>[2x]GAMDPEFALQELRAQHEDQVEQYKKELEKTYSAKLDNARQSAERNSNL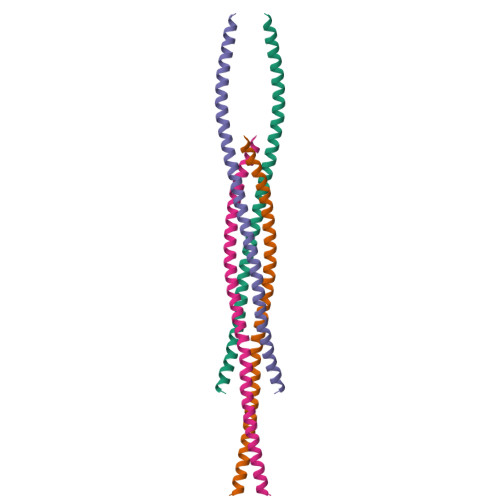VGAAHEELQQSRIRIDSLSAQLSQLQKQLAACEAKLRDLEDSLARERDTSRRLLA> KEKH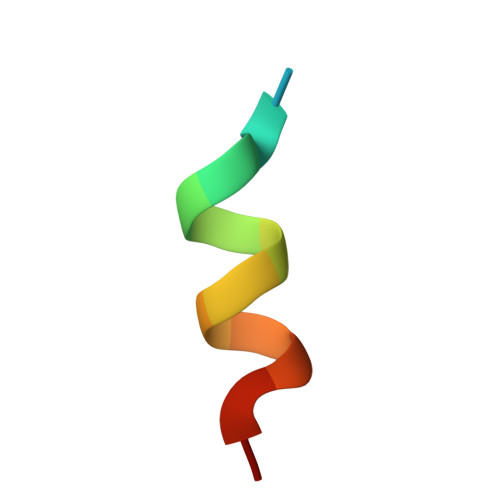KILHRLLQDSS The PRV capsid, similar to other herpesviruses, has a triangulation (T) number of 16 and is composed of major capsid proteins (MCPs), small capsid proteins (SCPs), and triplexes. The MCP (VP5) is encoded by UL19 and forms pentamer (penton) and hexamer (hexon) in the capsid. The hexon MCP is decorated with the SCP (VP26 protein, encoded by UL35), whereas the penton MCP lacks decoration. The triplexes, each composed of one VP19C protein (Tri1, encoded by UL38) and two VP23 proteins (Tri2, encoded by UL18), anchor to the capsid floor via Tri1 N-anchor.

Here, we use cryo-EM to image both the PRV empty capsid resulted from abortive DNA packing (A-capsid) and mature capsids fully packed with DNA (C-capsid). From the same dataset, we selected a total of 14,252 and 8899 particles for PRV C-capsid and A-capsid, respectively, and, by imposing icosahedral symmetry, obtained three-dimensional (3D) reconstructions at resolutions of 4.43 and 4.53 Å, respectively. Local reconstructions were then carried out to finally obtain the cryo-EM structures of the C-capsid 5-, 3-, and 2-fold sub-regions at 3.31, 3.46, and 3.43 Å, respectively, and the A-capsid 5-, 3-, and 2-fold sub-regions at 3.64, 3.50, and 3.41 Å, respectively. Five CATCs form a star-shaped tegumental layer that is situated on both the penton and portal vertices, forming extensive interactions with the penton and portal proteins to stabilize the conformation of the vertex complexes. Like other herpesviruses, each CATC of PRV bridges the space between the penton/portal and hexon by binding at two triplexes, Ta and Tc. Based on our localized reconstruction of the C-capsid 5-fold sub-particle, an atomic model of PRV CATC was built; however, only the N-terminus of the pUL25 subunits (upper pUL25 aa 1-73; lower pUL25 aa10-83) could be built out as α-helices; the remaining C-terminal globular domain, in contrast, was disordered and failed to be modeled. A comparison of the penton and portal vertexes also revealed a slight difference (~6°) in the orientations of the bound CATCs; such discrepancies may influence their interactions with the triplexes underneath. Indeed, we observed that the peri-portal Triplex Ta rotates counterclockwise by ~120° when compared to peri-penton Ta. The portal-containing capsid reconstruction revealed an ordered, layered dsDNA around a less-ordered core.

>MERPAILPSGQILSNIEVHSHRALFDIFKRFRSDDNNLYGAEFDALLGTYCSTLSLVRFLELGLSVACVCTKFPELSYVAEGTIQFEVQQPMIARDGPHPADQPVHNYMIKRLDRRSLNAAFSIAVEALGLISGENLDGTHISSAMRLRAIQQLARNVQAVLDSFERGTADQMLRVLMEKAPPLSLLAPFTLYEGRLADRVACAALVSELKRRVRDDTFFLTKHERNKDAVLDRLSDLVNCTAPSVAVARMTHADTQGRPVDGVLVTTAGVRQRLLHHVLTLADTHADVPVTYGEMVIANTNLVTALVMGKAVSNMDDVARYLLGGEPAPDDGKPVGSARVRADLVVVGDRLVFLEALEKRVYQATQVPYPLVGNLDVTFVMPLGVFKPAADRYARHAGSFAPTPGLPDPRTHPPRAVHFFNKDGVPCHVTFEHAMGTLCHPSFLDVDATLAALRQEPAEVQCAFGAYVADARPDALVGLMQRFLEEWPGMMPVRPRWAAPAAADQLLAPGNADLRLELHPAFDFFVAPEVDVPGPFAVPQVMGQVRAMPRIINGNIPLALCPVDFRDARGFELSVDRHRLAPATVAAVRGAFRDANYPMVFYIIEAVIHGSERTFCALARLVAQCIQSYWRNTHNAAFVNNFYMVMYINTYLGNGELPEDCAAVYKDLLEHVHALRRLIGEFTLPGDPLGNQPQEELNHALADATLLPPLIWDCDPILYRDGLAERLPELRVNGAHFQHILWVEMAQVNFRNVGGGLVHNRPVRNENQPLHPHHDAEWSVLSKIYYYAVVPAFSRGNCCTMGVRYDRVYQLVQTMVVPETDEEVGTDDPRHPLHPRNLVPNSLNVLFHNACVAVDADAMLILQETVTNMAERTTPLLASVAPDAGMATVATRDMRTHDGSLHHGLLMMAYQPNDATLLEGAFFYPAPVNALFACADHLGAMRDVGAEVRAAAQHVPCVPHFLGANYYATVRQPVAQHAAQSRADENTLSYALMAGYFKMSPVAFTHQLRRQLHPGFALTVVRQDRFATENVLFAEKASESYFMGQMQVARTESGGGLHLQLTQPRANVDLGVGFTAAYAAAALRAPVTDMGNLPQNLFATRGAPPMLDADADDYLRRTVNAGNRLAPVPVFGQMLPQVPAGLARGQQSVCEFIATPVSVDLAYFRRACNPRGRAAGEVHGEEGLMFDHSHADPAHPHRATANPWASQRHSYADRLYNGQYNMSGPAYSPCFKFFTPAEAVAKSRGLARLIADTGAAASPTSNGEYQFKRPVGAGELVEDPCALFQEAYPPLCASDSALLRTPLGAEEHFAQYLIRDESPLKGCFQHASA[16x];>[10x]MEVDIALPTLSPGDLSALQRCEGRVVFLETLRRHATLREVALPCGGDVLAAMAAYRRRFAAVITRVTPHRMLATPLGVGGRGQSLVLQNTGPFDLTNGDHVCLVPPLLGDECLRLTSANLELRFPMTLPLAQARELTARVVARAAETLRGGAPARGADVVFSNGRRYQLPPPHRDNAEAATRSLVLNMIFLLNEGAVILLSLIPNLLTLGAQDGYANAVIQLGSATRELGQLVRQPPPPLPQDHARRFCVFEALEAWIASASRLGDTLGTRPVARVCIFDGPPTVPPGEKAAVVEV;> MDAHIANETKQQMTRFAPALVHVIVPDPLLARAGVDPLAPFAAHAQTRYHGSGVCEPWVSVFAGHVQTGAVESVLTLPPLQRPRGPGGLFVSLPLALGAHFDGFTTAALRVGARELVFTYDELLPARTRYNVDGERLERLCRQFANYARARRVAPAVAAAGGHIDALLPPAAATIDGEAQLTRGGFDDPAAPHARDADREILSLVRRAAELVAARHPVRSHVASGLMQGALARRGGGGDGAGALEAAATVPAPAAREDANGGGAAWRDELLLTPQDPRPLTALDWLDAGYAALAGGDAPAHVWRRRPVSLVARRHYQTGETFVVVAYEHSTAWGGRRGPRGEPLARVLAEECERHGVEHPRALPAEARRELVRRHAELAVPLGDEEPPLPVFDATAELVLLERFRNACVRALLAGVRESVRREPRMRQIIEFAIRPRDREAVLDVAGRAPALLDAFARRLEHTPAREMVDSGLMTAAAAHLAARATAGYVTFESGPLLGGVFLFDYYSAGGEVIRVTRAPLAVAVEPATRGQFACRFRGASHRCLPGESYAYLCVGVSRDLRALVVLPGGFGFFATLRLEWPAALVDPVLERLCRRV;>[15x]MSFDPNNPRTITAQTLEGALPVDILLRLNRATGLQMDAAEAHAIVEDARRTLFIGTSLALVNLRRAHDKHLVERQPMFATSDYSSWARPTVGLKRTFCPRPPP;>[5x]MSVQIGNGLLMVVAPGTLTVGSARARLIRQVTLADFCEPQAERPGLVVLALRHPADLAGAAYAATPPGKNHRDLEEAWLALDEGGRGLGGDGIRASVVSLNFLVAAAENADDALRAHVTTNYRDRRTAARLERFATVLRAMIRSHVFPHRALHVLGGLLGHVTQDRLASVTCVARGDQEAARTNDMAARRSQVHVPACALMDVDRELRLGGDDGLRFAYLVFVYTQRHRREALRVHVAVSRLPELGDALSFLLAGTRVDNAIHGTDEADAPAAPAAAAAFPAYLFNDPRSARCPTGRLNTPAAEALPVWAPDMRGRATRNSCMYAAYVRLGTVERVVRRAERCGSVDLPLAHMERFTWDVGAWEECFF;>[2x]MDRAWFAFEAAAIPGSARHFIAPPFPVGFWARPGFGEGLDARLALAHANARRRAAAAALDNAMAAGARLEAEVDEQLRPLERQVERVAEALVVLEETARAAEEADAARAAEEAPEATAAADEGREVQIAKNDVALAYDANLSLDFLAMVYAARGAASGVLFGTWYATLQATLVAERPQVSRAIDSRDGRMSRTFMGVTTTALQACGRLYVGNRHYSALESAALCLHLVHRARQGPGAAGAAAPLGIADLLERVPEYLDALSQALAEGGRISYRYNYARVPREQLHGRYALEGHSVLAALARLRVVPGANVGANEVDGAGFVDEVNRAAAAFLGRGQNLFLGEDAPLLRATVNTITGLLLLRRLLHNGNVYGDRLRNNFQLGALVPNAPPPRGASGDAPASRSGDGNLRFLLAHYVVVAYRADERTELTQLFPGLAALALDAHSIRARVQRHQLNLVRLVALELQNRQRVTAPVNEVIAAHDAVAVQYEEGLGLLLQQPHLRNAADKRLGQFGVSSDYDLLYFLCLGYIPQFAAA;>RVVESDTLINRRYMRATGLGALALLIAACRLIARRLRETRTTLKGSARRFNVDLFQVRLILG[2x]> MSFKATITESGKQNIWFRAIYVLSTIQDDIKITVTTNELIAWSMNETDTTLCQVRFQKSFFEEYEFKPHEIVFGENGVQVIEDTYGNSHKLYSFRVNGRHLTTISRKPDGDGIKSFTIAVNNTSTCPESLANRLIVVIEMDSLIVKEYCPQFQPIKYDPIIINLKYKRRFLDVFGTAASDRNPQEPLDPKLLDVFTNTERELTSALFNEEVESDIRKRNQLTAADEINYICCNSTLLKNFLDNCNVNVTDEVKLEINVHRLSITAFTKAVYGKNNDLLRNALSMSNTISTLDLEHYCLFTKSIIFKLKDFKNFITIGPSWKTTQDGNDNISLWFCHPGDPILMQMQKPGVKLELVEVTDSNINDDILEGKFIKTAISGSKEEAGLKDNKES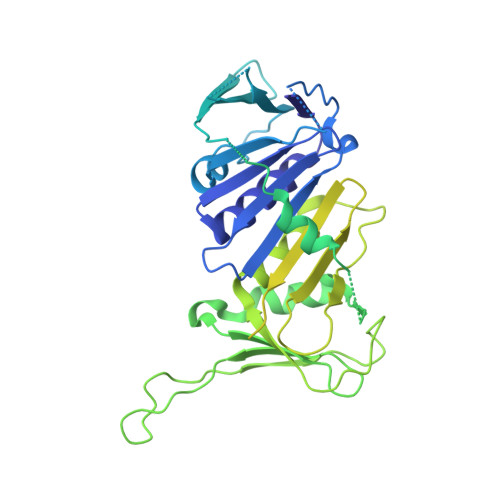CESPLKSKTALKRENLPHSVAGTRNSPLKVSYLTPDNGSTVAKTYRNNTARKLFVEEQSQSTNYEQDKRFRQASSVHMNMNREQSFDIGTTHEVACPRNESNSLKRSIADICNETEDPTQQSTFAKRADTTVTWGKALPAADDEVSCSNIDRKGMLKKEKLKHMQGLLNSQNDTSNHKKQDNKEMEDGLGLTQVEKPRGIFD> APIPGVMPIGNYVSLYVMLPLGVVNADNVFPDKEKVEDELKQVKAGGCDGVMVDVWWGIIEAKGPKQYDWSAYRELFQLVKKCGLKIQAIMSFHQCGGNVGDAVFIPIPQWILQIGDKNPDIFYTNRAGNRNQEYLSLGVDNQRLFQGRTALEMYRDFMESFRDNMADFLKAGDIVDIEVGCGAAGELRYPSYPETQGWVFPGIGEFQCYDKYMVADWKEAVKQAGNADWEMPGKGAGTYNDTPDKTEFFRPNGTYKTDMGKFFLTWYSNKLIIHGDQVLEEANKVFVGLRVNIAAKVSGIHWWYNHVSHAAELTAGFYNVAGRDGYRPIARMLARHHATLNFTCLEMRDSEQPAEAKSAPQELVQQVLSSGWKEYIDVAGENALPRYDATAYNQMLLKLRPNGVNLNGPPKLKMSGLTYLRLSDDLLQTDNFELFKKFVKKMHADLDPS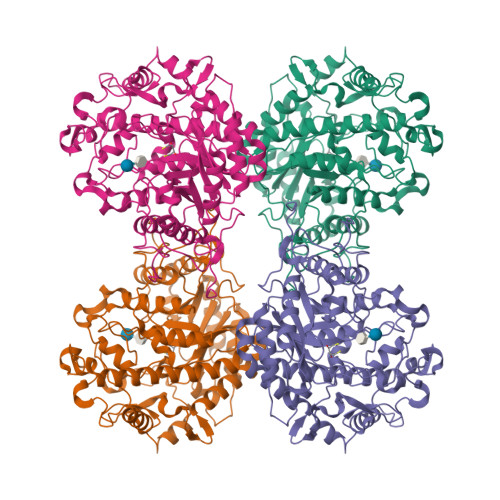PNAISPAVLERSNSAITIDELMEATKGSRPFPWYDVTDMPVDGSNPFD> NEAIECHLSDLLQQLTSVNASKPSERGLVRQEEAEDPACIPIFWVSKWVDYSDKYGLGYQLCDNSVGVLFNDSTRLILYNDGDSLQYIERDGTESYLTVSSHPNSLMKKITLLNYFRNYMSEHLLKAGANITPREGDELARLPYLRTWFRTRSAIILHLSNGTVQINFFQDHTKLILCPLMAAVTYINEKRDFQTYRLSLL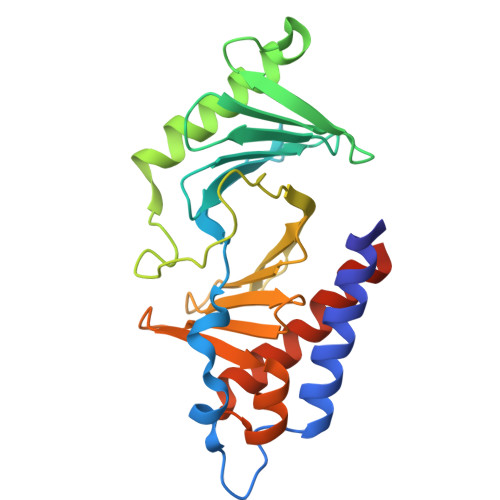EEYGCCKELASRLRYARTMVDKLLSSRSASNRLKAS> MNDKEKIDKFIHSNLNDDFGLSVDDLVGKVKGIGRFSAWCGNSSTKIKQVLNAVKSIGVSPALFAAYEKNEGYNGSWGWLNHTSPQGNYLTDAQFVARKLVSQSRQAGTPSWIDAGNPVDFVPASVKRKGNYDFSHNMKNGKVGRAYIPLTAAATWAAYYPEGLQASYNRVQNYGNPFLDAANTILGWGGKIDGKGGSSSGSSSSSSGTSGGLDVVARAFEEFLKKLQDSMQWDLHSIGTDKFFSNQMFTITKTYNNTYRLNMNQKLLDEMKDLISRIDGGSGNDTGADDSDGDHGGKAGKSVAPNGKSGRKIGGNWTYSNLPQKYKDAIEVPKFDPKYLAGSPFVNTGDTGQCTELTWAYMHQIWGKRQPAWDNQVTNGQRVWVVYRNQGARVTHRPTVGYGFSSKPNYLQAMLPGVGHTGVVVAVFKDGSFLTANYNVPPYWAPSR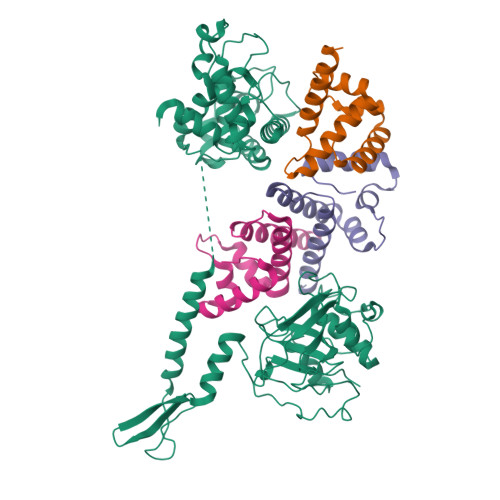VVEYALIDGVPENAGDNIMFFSGIK;>[3x]VTNEKGQAYTEMLQLFNLLQQWNDFYTAENANNLLVACQQLLINYNEPVIKFINDENEDKSLLQYLAGDDGLAQWQFYKGFYNNYNVHIF> MRGSHHHHHHTDPHEEENDVVKGNFDISKISGDWYSILLASDIKEKIEENGSMRVFVKDIEVLSNSSLIFTMHTKVNGKCTKISLICNKTEKDGEYDVVHDGYNLFRIIETAYEDYIIFHLNNVNQEQEFQLMELYGRKPDVSPKVKEKFVRYCQGMEIPKENI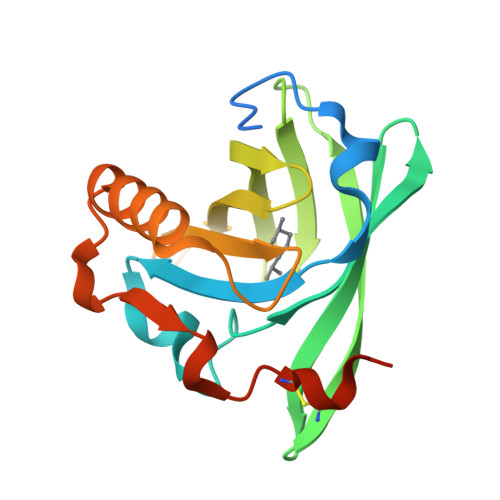LDLTQVDRCLQARQSEAAQVSSAE>MKKILIIGGVAGGASAAARARRLSETAEIIMFERGEYVSFANSGLPYHISGEIAQRSALVLQTPESFKARFNVEVRVKHEVVAIDRAAKLVTVRRLLDGSEYQESYDTLLLSPGAAPIVPPIPGVDNPLTHSLRNIPDMDRILQTIQMNNVEHATVVGGGFIGLEMMESLHHLGIKTTLLELADQVMTPVDREMAGFAHQAIRDQGVDLRLGTALSEVSYQVQTHVASDAAGEDTAHQHIKGHLSLTLSNGELLETDLLIMAIGVRPETQLARDAGLAIGELGGIKVNAMMQTSDPAIYAVGDAVEEQDFVTGQACLVPLAGPANRQGRMAADNMFGREERYQGTQGTAICKVFDLAVGATGKNEKQLKQA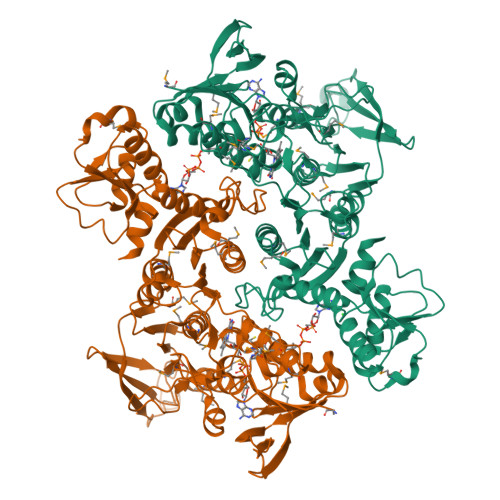GIAFEKVYVHTASHASYYPGAEVVSFKLLFDPVKGTIFGAQAVGKDGIDKRIDVMAVAQRAGMTVEQLQHLELSYAPPYGSAKDVINQAAFVASNIIKGDATPIHFDQIDNLSEDQLLLDVRNPGELQNGGLEGAVNIPVDELRDRMHELPKDKEIIIFSQVGLRGNVAYRQLVNNGYRARNLIGGYRTYKFASVLEHHHHHH[2x]>[2x]SEWLTDFIIDALDSGRFWGVGW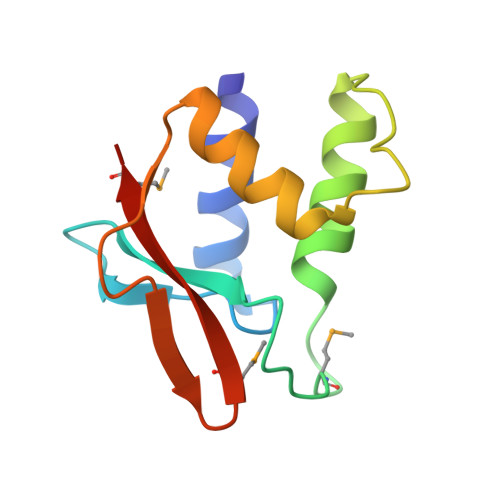LDEQKRIFTVPGRNRRERMPEGFDDFYEAFLEERRRHGLPEIPETETGLGCFGRLLRTANRARQERPFTIYKGKMKLNRWIMTPRP>ADPGHHHHHHGGCPSQCSCSGTTVDCRSKRHASVPAGIPTNAQILYLHDNQITKLEPGVFDSLINLKELYLGSNQLGALPVGVFDSLTQLTVLDLGTNQLTVLPSAVFDRLVHLKELFMCCNKLTELPRGIERLTHLTHLALDQNQLKSIPHGAFDRLSSLTHAYLFGNPWDCECRDIMYLRNWVADHTSIA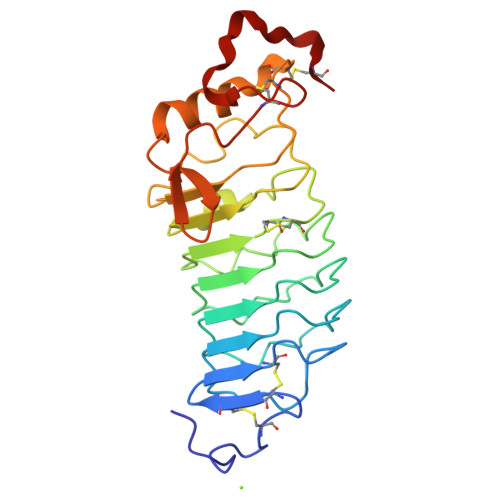MRWDGKAVNDPDSAKCAGTNTPVRAVTEASTSPSKCP[2x]(4-chloropyridin-2-yl)methanol | C6 H6 Cl N O | 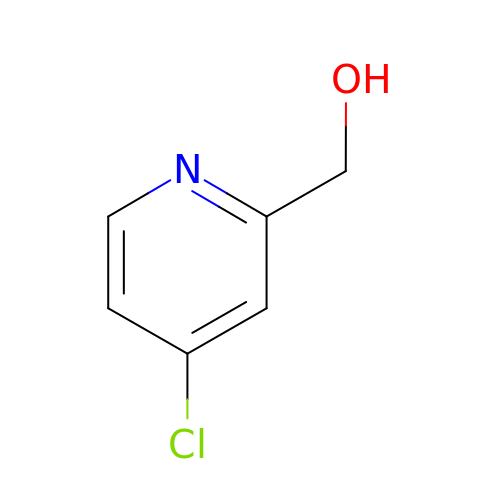UEAIOHHGRGSGGJ-UHFFFAOYSA-N> MDVHIDNQVLSGLGTPLLVHLFVPDTVMAELCPNRVPNCEGAWCQTLFSDRTGLTRVCRVFAARGMLPGRPSHRGTFTSVPVYCDEGLPELYNPFHVAALRFYDEGGLVGELQIYYLSLFEGAKRALTDGHLIREASGVQESAAAMQPIPIDPGPPGGAGIEHMPVAAAQVEHPKTYDLKQILLEITQEENRGEQRLGHAGSPALCLGLRLRAGAETKAAAETSVSKHHPALENPSNIRGSAGGEGGGGRAGTGGTVGVGSGALSRVPVSFSKTR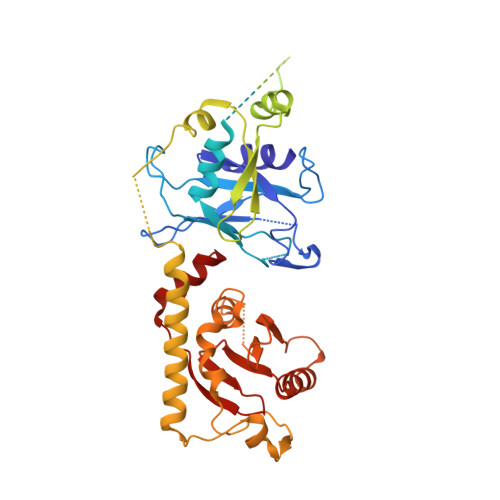RAIRESRALVRGIAHIFSPHALYVVTYPELSAQGRLHRMTAVTHASPATDLAEVSILGAPEREFRFLISVALRISASFREKLAMQAWTAQQEIPVVIPTSYSRIYKNSDLIREAFFTVQTRVSWESCWVKATISNAPKTPDACLWIDSHPLYEEGASAWGKVIDSRPPGGLVGAASQLVALGTDGHCVHLATTSDGQAFLVLPGGFVIKGQLALTPEERGYILARHGIRREQ Type IV pili (T4P) are functionally versatile filaments widespread in prokaryotes, composed of type IV pilins and assembled by conserved multiprotein machineries. We show that PilB is a modular pilin with a bulky module “grafted” onto a small pilin module, which directly mediates adhesion of S. sanguinis to host cells/proteins. PilB, one of the three minor pilins in S. sanguinis T4P, exhibits a canonical N-terminal class III signal peptide, the defining feature of type IV pilins. The larger size of PilB is due to the presence of a C-terminal domain readily detectable by bioinformatics, which belongs to the von Willebrand factor A–like domain superfamily (InterPro entry IPR036465).

To confirm that metal binding involves the MIDAS motif, we produced PilBD319A in which the key MIDAS residue Asp319 was changed into an Ala by site-directed mutagenesis. Binding assays performed with PilBD319A showed that changing this single residue abolishes the metal-binding ability of PilB for both Mg2+ and Mn2+. Next, to determine whether metal presence/absence might impact the 3D structure of PilB, we solved the structure of PilBD319A by X-ray crystallography. The PilBD319A protein readily crystallized in the same condition as the wild-type (WT) protein. We collected a complete dataset on crystals diffracting to a resolution of 3 Å and solved the structure of PilBD319A by molecular replacement. The structure of PilBD319A clearly shows that no metal is occupying the mutated MIDAS pocket on top of the central β-sheet, which is consistent with metal-binding assays. Although PilBD319A resolution is significantly lower than WT, it nevertheless allows for meaningful structural comparison. When the vWA modules were compared, we found that they are essentially identical, the Cα atoms superposing onto each other with an RMSD of merely 0.45 Å, including the two arms flanking the MIDAS pocket. This shows that metal binding by MIDAS has no detectable structural impact on PilB.

>[2x]SSRELIEREASIQAEMRTSMQYVDRTVGKATSIFILDDSKFKGSKQGLTREWSYIGLSADGKKVMNYVWNKQKQDWDVSELGTKSLYNMKLDLEFKTEGAYQDNRLISYNLTGKYPDTNNKLGIDTAISALNTKQVFSKVAKGKKGIAIAYRTDPIQGQMNIAVSFVFDTSGSMDWDLQGRNVKKTGNESRMDILRKKSVIMIKDLAEIGNISVNLVGFSTSAKYIQQNFSNLDNGTNTIIATITKRENLNPDGVTNPGDGLRYGMISLQSQPAQLKYIVLLTAGIPNAYLVDSRALYAGNRVDLSQGAGRVTFNNPIYDLSPTLGYEYSRLGYDLYSRDSITRENSIAYAGEVSKKFGLGIKRVNVIGFSGVNHEIAYGQSLTDRIGEGGMETKYVSATNEEALQKTFSDIKKQIQQDLWFVSGP> SLKVLAITGYKPFELGIFKQDDKALYYIKKAIKNRLIAFLDEGL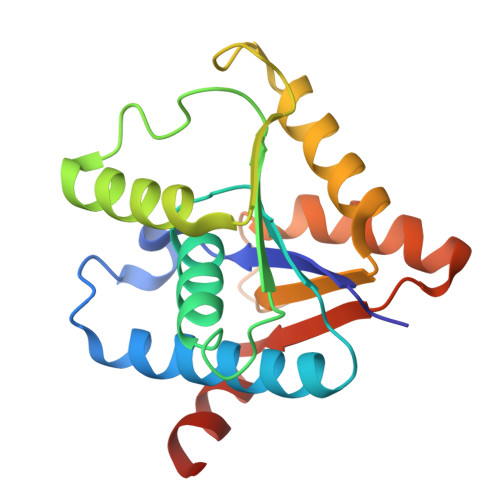EWILISGQLGVELWAAEAAYDLQEEYPDLKVAVITPFYEQEKNWKEPNKEQYEAVLAQADYEASLTHRPYESPLQFKQKNQFFIDKSDGLLLLYDPEKEGSPKYMLGTAEKRREQDGYPIYFITMDDLRVTVEEDSY1-[3-CYANO-4-(NEOPENTYLOXY)PHENYL]-1H-PYRAZOLE-4-CARBOXYLIC ACID | C16 H17 N3 O3 | 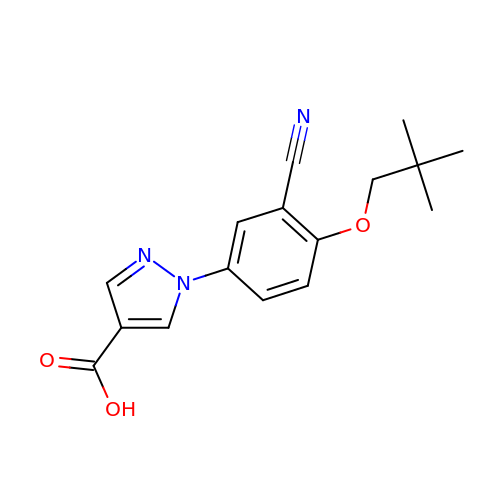AETHRPHBGJAIBT-UHFFFAOYSA-N>LTLWTTPDPSPNCTIDQERDSKLTLVLTKCGSQILANVSLLVVKGKFSNINNNTNPTDKKITVKLLFNEKGVLMDSSTLKKEYWNYRNDNSTVSQAYDNAVPFMPNIKAYPKPTTDTSAKPEDKKSAAKRYIVSNVYIGGLPDKTVVITIKFNAETECAYSITFEFTWAKTFEDVQFDSSSFTFSYIAQENEDEDK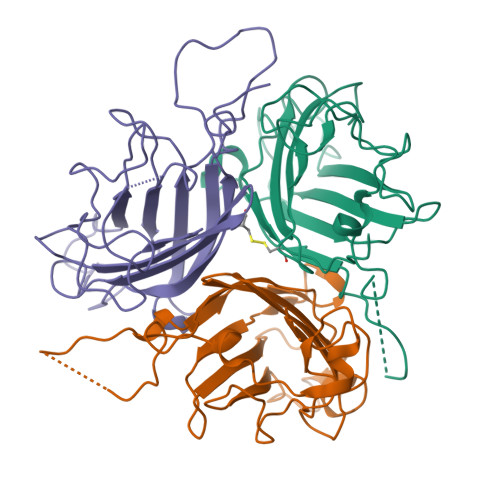[6x]>[2x]MRVLLSVCGTRGDVEIGVALADRLKALGVQTRMCAPPAAEERLAEVGVPHVPVGLPQHMMLQEGMPPPPPEEEQRLAAMTVEMQFDAVPGAAEGCAAVVAVGDLAAATGVRSVAEKLGLPFFYSVPSPVYLASPHLPPAYDEPTTPGVTDIRVLWEERAARFADRYGPTLNRRRAEIGLPPVEDVFGYGHGERPLLAADPVLAPLQPDVDAVQTGAWLLSDERPLPPELEAFLAAGSPPVH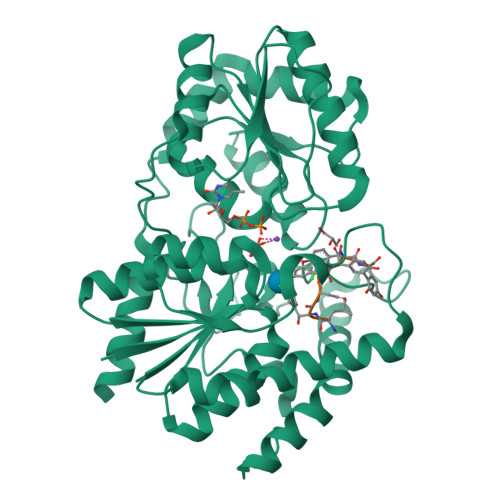IGFGSSSGRGIADAAKVAVEAIRAQGRRVILSRGWTELVLPDDRDDCFAIDEVNFQALFRRVAAVIHHGSAGTEHVATRAGVPQLVIPRNTDQPYFAGRVAALGIGVAHDGPTPTFESLSAALTTVLAPETRARAEAVAGMVLTDGAAAAADLVLAAVGREKPAVPALEHHHHHH> VVQAPTQVPGFLGDSVTLPCYLQVPNMEVTHVSQLTWARHGESGSMAVFHQTQGPSYSESKRLEFVAARLGAELRDASLRMFGLRVEDEGSYTCLFVTFP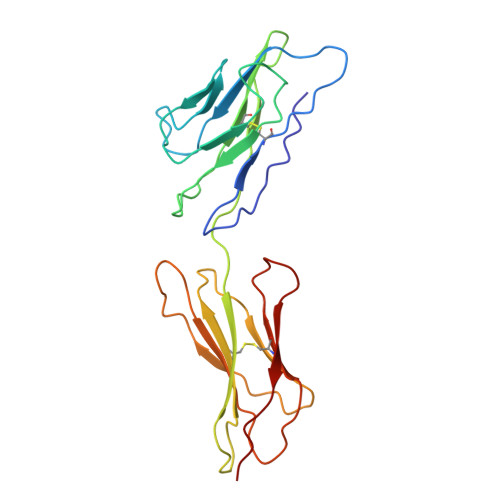QGSRSVDIWLRVLAKPQNTAEVQKVQLTGEPVPMARCVSTGGRPPAQITWHSDLGGMPQTSQVPGFLSGTVTVTSLWILVPSSQVDGKQVTCKVEHESFEKPQLLTVSLTVYY>[2x]SQVTEQSVRFQTALASIKLIQASAVL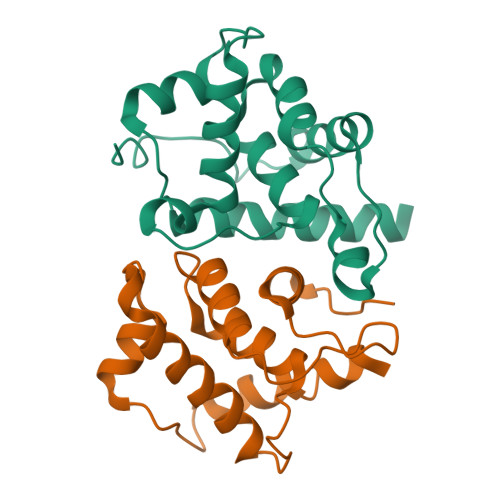DLTEDDFDFLTSNKVWIATDRSRARRCVEACVYGTLDFVGYPRFPAPVEFIAAVIAYYVHPVNIQTACLIMEGAEFTENIINGVERPVKAAELFAFTLRVRAGNTDVLTDAEENVRQKLRAEGVM> ADAPAGTDPRAKWVPQDNDIQACDYWRHCSIDGNICDCSGGSLTNCPPGTKLATASWVASCYNPTDGQSYLIAYRDCCGYNVSGRCPCLNT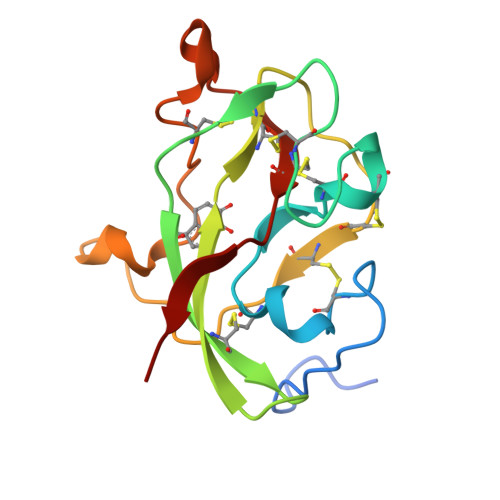EGELPVYRPEFANDIIWCFGAEDDAMTYHCTISPIVGKAS> MNWSKAINFQPFMLETRPPLTTIPIMDQLVEIGERSNQKWSMTDRLFFAIRKINPIFVTSSQIPSKFDYTILQMPTQLIASLKETLLFLAFSYYLREYQDKVGQMKFYPVAMKNMIPIVNYLKDRVHNNFDTTLEQAYRQNVVHTLSASDAFDLLSGMIATTRLDLIQRT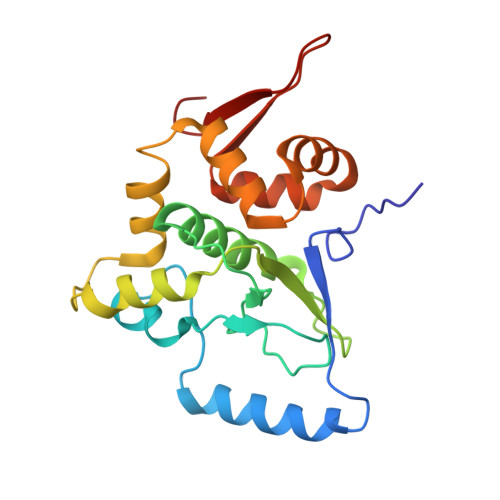RICPELLNVLNKMSFILIYAPNRPSILSWKNQS2-bromanyl-N-(5,6,7,8-tetrahydro-[1]benzothiolo[2,3-d]pyrimidin-4-yl)benzamide | C17 H14 Br N3 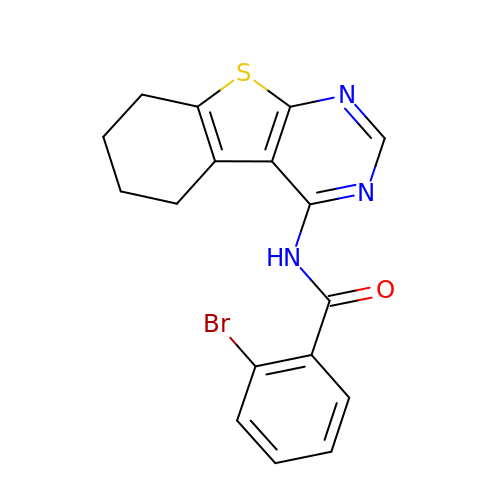O S | KFSLRFWIPVMBNT-UHFFFAOYSA-N> GGVDREAMARCIEECLRCAQACTACADACLSEPTVADLTKCIRTDMDCADVCTATAAVLSRHTGYDANVTRAVLQACATVCAACGDECARAAGMAEHCRVCAEACRSCEQA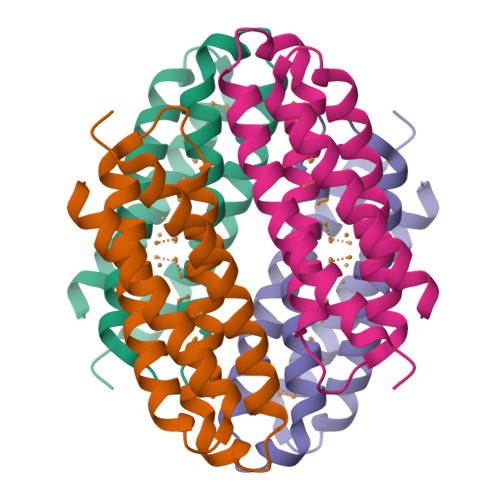CQELLAGL>MRIYVLGAGSIGSLFGALLARAGNDVTLIGRREQVDAINKNGLHVFGAEEFTVKPKATIYAPEEPPDLLILAVKSYSTKTALECARQCIGRNTWVLSIQNGLGNEELALKYTPNVMGGVTTNGAMLVEWGKVLWAGKGITVIGRYPTGRDDFVDEVASVFNEAGIDTSVTENAIGWKWAKAIVNSVINGLGTVLEVKNGHLKDDPHLEGISVDIAREGC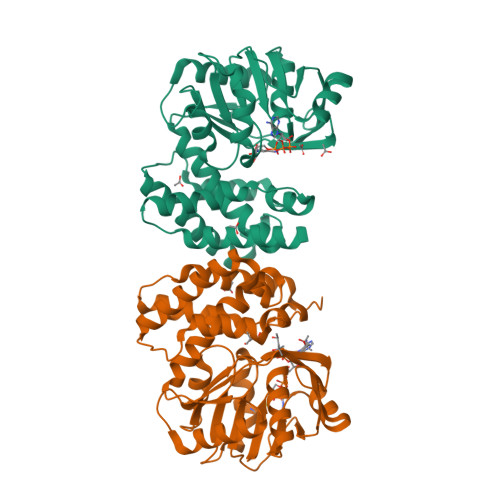MVAQQLGIEFEIHPLELLWDTIERTRENYNSTLQDIWRGRETEVDYIHGKIVEYARSVGMEAPRNELLWVLVKAKERINRGKTRNISEGC[2x]> TTIVA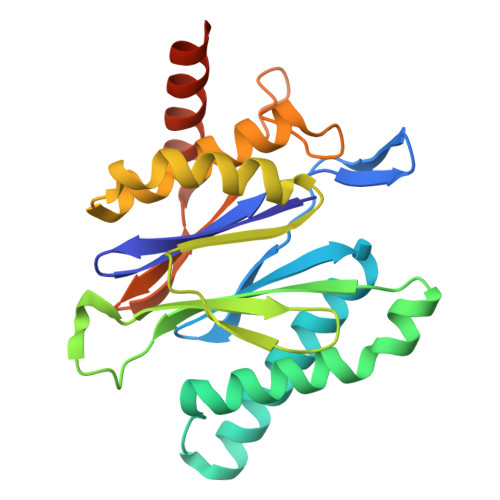LKYPGGVVMAGDRRSTQGNMISGRDVRKVYITDDYTATGIAGTAAVAVEFARLYAVELEHYEKLEGVPLTFAGKINRLAIMVRGNLAAAMQGLLALPLLAGYDIHASDPQSAGRIVSFDAAGGWNIEEEGYQAVGSGSLFAKSSMKKLYSQVTDGDSGLRVAVEALYDAADDDSATGGPDLVRGIFPTAVIIDADGAVDVPESRIAELARAIIESRSGADTFGSDGGEK>MINFPKPTVEQFFRTYTITNFAVSSDEKRLVFNANLNGKMNLWAMDLPDTYPYLFAHRDESCNFIKFDPENRYVLAGFDKDGDENYQIYAIPNEGGLPHPLITGDASEKYYFSHLSADGKCVYYETSKENPSFLNTRIRNLETGEDRLLNVGEVSTTELAAVSENEESFVYLRAFANTYIVGFVKMGEETFNITPDPEKVHVAMEPVFTDNETIYFATDYDSDEMYLAKFDLTSKEFSKVLAFDGESIQSVKWDKDNKAFYLITVKGVTDILYRYDVATDKVEECSLPVDIIEQIQVAKSGNLYILGRSATVPHNVYQSSNGVEWKQLTNNRVLGLSPEDMVEPDIVSYTSFDGMEIEALLFKAKPENDNGYTIFWPHGG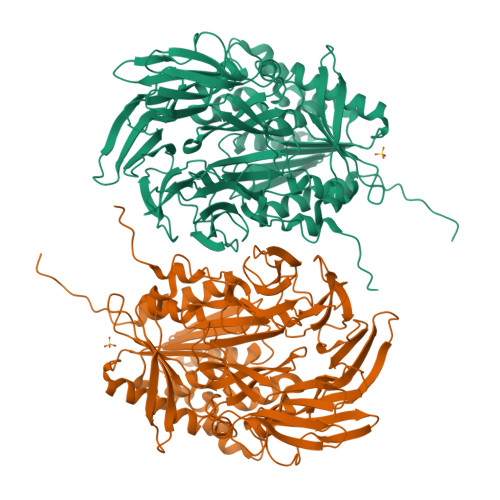PQSAERKMFRSMFQCFINRGYTIFAPNFRGSTGYGSAFTKLVELDWGEGPRLDCIAGIEWLFESGFTDRNKLFLVGGSYGGYMALLLHGRHSDYFRAVVDIFGPSDLFTFINSVPPHWKPIMERWLGDPERDKERFIKDSPVTYLDGMVKPMLVIQGAKDPRVVKEESDQIVAKLKEKGRDVEYLVLEDEGHGFSKKENEIKVYSLMLAFLEKHQALEHHHHHH[4x]> LAPRKQ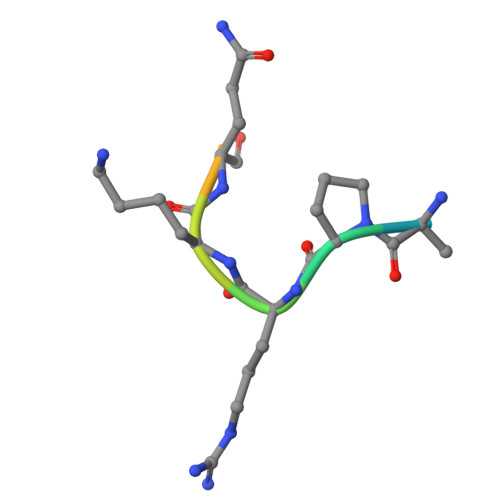LATK>MASMTGGQQMGAPITAYAQQTRGLLGCIITSLTGRDKNQVEGEVQIVSTATQTFLATCINGVCWTVYHGAGTRTIASPKGPVIQMYTNVDQDLVGWPAPQGSRSLTPCTCGSSDLYLVTRHADVIPVRRRGDSRGSLLSPRPISYLKGSSGGPLLC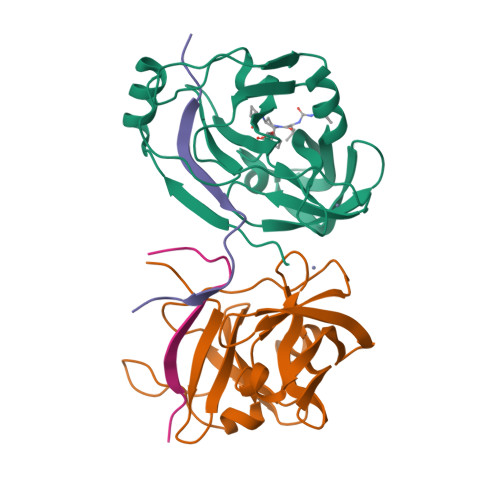PAGHAVGLFRAAVCTRGVTKAVDFIPVENLETTMRSGSHHHHHH[2x];>KKGSVVIVGRIVLSGKPAIIPKK[2x]> MNIKTLLLITSAIFISACSPYIVTANPNHSASKSDEKAEKIKNLFNEVHTTGVLVIQQGQTQQSYGNDLARASTEYVPASTFKMLNALIGLEHHKATTTEVFKWDGQKRLFPEWEKDMTLGDAMKASAIPVYQDLARRIGLELMSKEVKRVGYGNADIGTQVDNFWLVGPLKITPQQEAQFAYK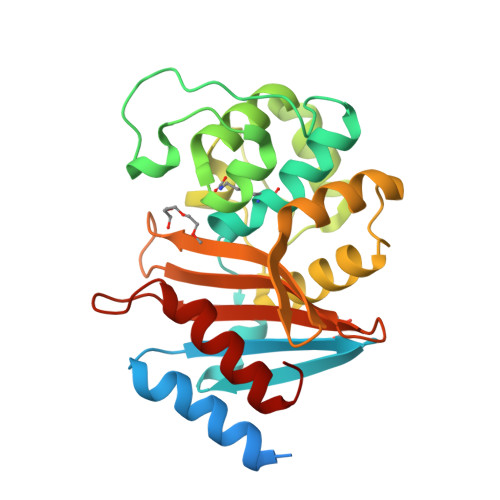LANKTLPFSPKVQDEVQSMLFIEEKNGNKIYAKSGWGWDVDPQVGWLTGWVVQPQGNIVAFSLNLEMKKGIPSSVRKEITYKSLEQLGIL(2R,3S,4S)-1-[(2S,3S,4R,5R,6S)-2,3,4,5,6,7-hexahydroxyheptyl]-3,4-dihydroxy-2-(hydroxymethyl)tetrahydrothiophenium (non-preferred name) 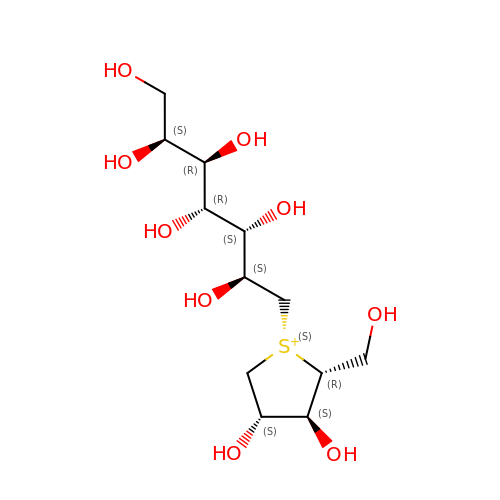| C12 H25 O9 S | JWOANRNVWBCYDC-RRTSSKPOSA-N> TNATGERNLALIQEVLEVFPETARKERRKHMMVSDPKMKSVGKCIISNRKSQPGVMTVRGCAYAGSKGVVFGPIKDMAHISHGPVGCGQYSRAGRRNYYTGVSGVDSFGTLNFT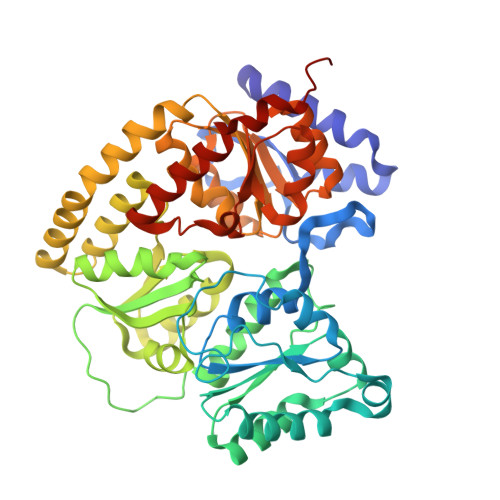SDFQERDIVFGGDKKLSKLIEEMELLFPLTKGITIQSECPVGLIGDDISAVANASSKALDKPVIPVRCEGFRGVSQSLGHHIANDVVRDWILNNREGQPFETTPYDVAIIGDYNIGGDAWASRILLEEMGLRVVAQWSGDGTLVEMENTPFVKLNLVHCYRSMNYIARHMEEKHQIPWMEYNFFGPTKIAESLRKIADQFDDTIRANAEAVIARYEGQMAAIIAKYRPRLEGRKVLLYMGGLRPRHVIGAYEDLGMEIIAAGYEFAHNDDYDRTLPDLKEGTLLFDDASSYELEAFVKALKPDLIGSGIKEKYIFQKMGVPFRQMHSWDYSGPYHGYDGFAIFARDMDMTLNNPAWNELTAPWLKSA> MKTEWPELVGKSVEEAKKVI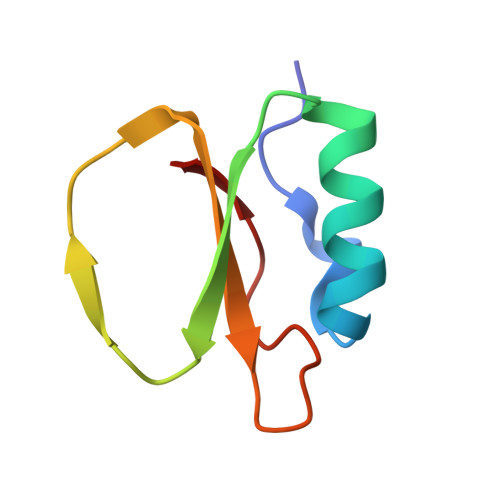LQDKPAAQIIVLPVGTIVTMEYAIDRVRLFVDRLDNIAQVPRVG> GPGSAEDVQQEAALLTKWQRIMGINYEIVVAHVSKFSENSGLGISLEATVG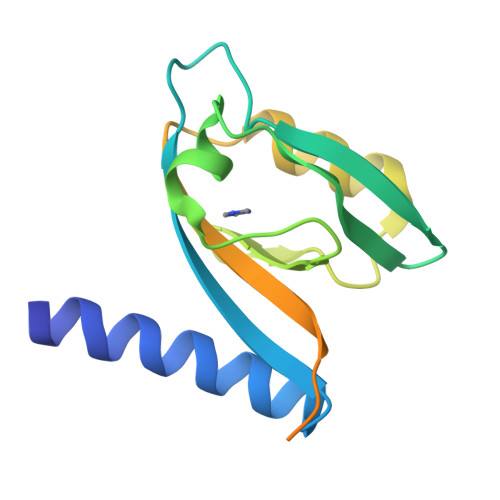HHFIRSVLPEGPVGHSGKLFSGDELLEVNGINLLGENHQDVVNILKELPIDVTMVCCRRTVPPIALSEMDSLDINDLELTEKPHIDLGEFIGSSETED> SNAENTDEDALMVTREDGSFLIDGTLPIEELREVLGAEL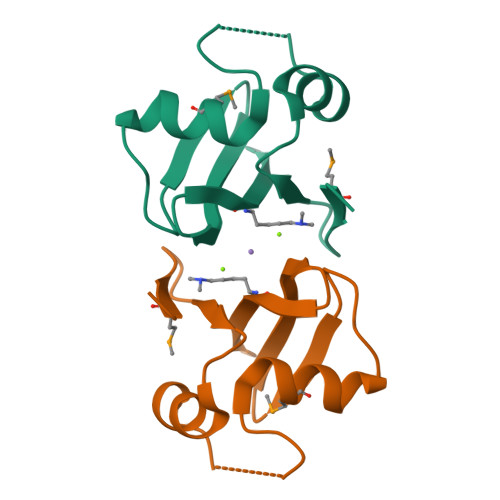PDGEENNYHTLAGMCISYFGRIPHVGEYFDWAGWRIEIVDLDGARIDKLLLQRLN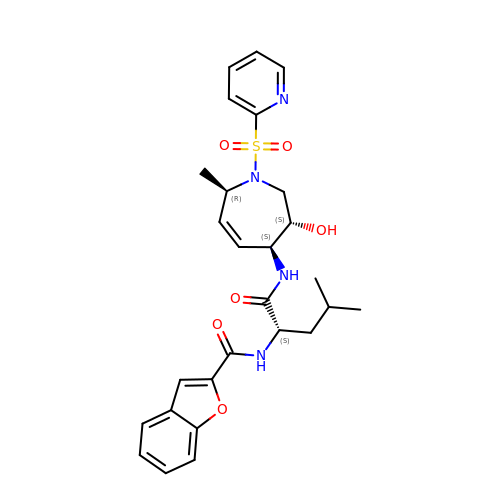N-[(1S)-1-({[(3S,4S,7R)-3-HYDROXY-7-METHYL-1-(PYRIDIN-2-YLSULFONYL)-2,3,4,7-TETRAHYDRO-1H-AZEPIN-4-YL]AMINO}CARBONYL)-3-METHYLBUTYL]-1-BENZOFURAN-2-CARBOXAMIDE | C27 H32 N4 O6 S | IJRITYSDIWFZKF-GBAJDQEWSA-N>GVLNQGVTSLESAKIDSVLPPLTVREASGVRTLSFGYDTSDFTIINSVLSLRSRLTLPTYRYPLELDTANNRVQVADRFGMRTGTWTGQLQYQHPQLSWRANVTLNLMKVDDWLVLSFSQMTTNSIMADGKFVINFVSGLSSGWQTGDTEPSSTIDPLS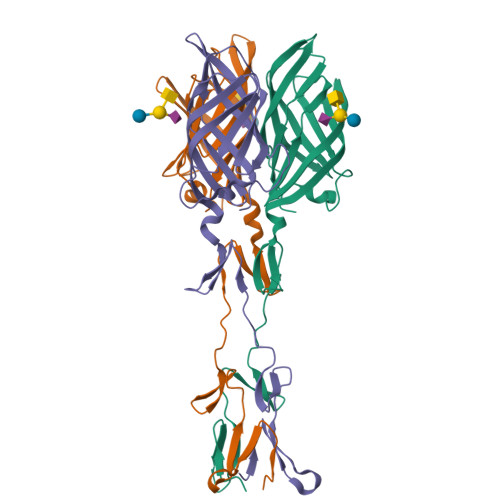TTFAAVQFLNNGQRIDAFRIMGVSEWTDGELEIKNYGGTYTGHTQVYWAPWTIMYPCNVR[3x]> MSATSGVVNRPLVLNHGSIESTILIPTTEYHFYQTLLEGFRKSLPQVTEGFADDDEPSSKAELLMKFLGYIVQSGVSNQQEQLAAAKLVLNEFESRFLQGLNLHSYAAILLKSETFPTTLLKIKENLIKNYYLGRALVYLPGQRGLVYPPSALLNAGKSGSAQIYAIFGGQGNTDDYFEELRDIYHIYQGLVSDFVTKAQLKLQELIRTTPETDRIYTQGLDLINWLENKDKTPDQQQLLSIPMSCPLICVIQLCHYIVTCRILGITPGQLRDSLKGTTGHSQGLVTAVVVSSADSWESFEKLALQAVEFMFYIGVRGLQTYPNTSLPPSIVQDSEENAEGTPSPMLSVRDLSYDQLVKFVNETNQHLPEAKHIDISLINGPRNVVLTGPPQSLYGLNLNLRKAKAPSGLDQARIPFSERKLRFSNRFLPIMSPFHSHLLSPSTEKIVADLKKAGVEFSQSSMKLPVFDTYDGKDLRSYSGSIAARLVECITKLRVNWELSTEFNSTHVLDFGPGGASGLGVLTHRNKEGTGSRVIVAGVLDAESEDSEFGYKQEIFESNEKAIKYAPNWLKEYKPKLVKTSAGKIFVDTKFSRLLGRAPLMVPGMTPTTVSPDFVAATLNAGFHTEIAGGGYFAPSIMKAALQRVIDQVTPGTGVGINLIYVNPRMLQWGIPMIKELREQGFPIQSLSIGAGVPSLEVATEYIETLGLAHLGLKPGSIDAVNQVITIAKAHPNFPIVLQWTGGRGGGHHSFEDFHQPILQMYSKIRKCKNIILIAGSGFGSAEDTYPYLTGSWSHQFSYPSMPFDGVLFGSRVMTAKEAKTSPAAKQAIADCTGVDNSQWENTYKKPTGGIITVRSEMGEPIHKIATRGVMLWKELDDTIFTLPKNKMLEAIAKKKDYIIKKLNADYQKPWFAKNEKGTCDLEDMTYKQIAERLVELMYVRKSQRWIDVTLRNFTGKFLRRIEERFATKVGTISLIQNFSQLEEPEKAIDSVFKAYPEAASQLINEEDCDWFLLEAQSPTQKPVPFIPVLDERFEFFFKKDSLWQSE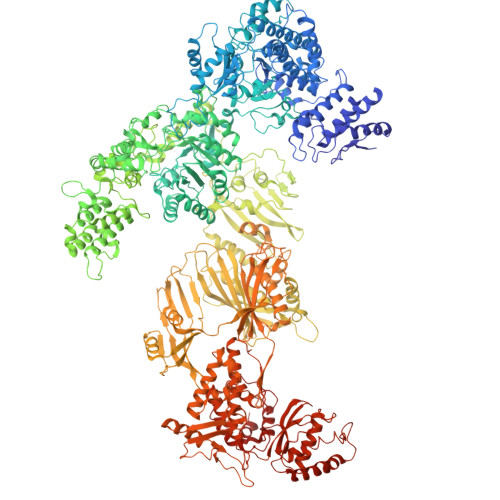DLEAVVGEDVQRTCILHGPVAAQFSNKVDEPIKDILENIHKGHIKSLVKEVYNGDESKIPVVEYFSSVDSFSDTAIEGVKIERSRNTETFTVTSGNVDNQQWFDLLAGKELSWRRAFITAARLVQGTNFVSNPAHSVLAPSKDLVVKIENGSDAKKTVLTAFQRVRGKYVPAVSLKSIGDLKIKLELIETRTADKSAVALELFYNYKPTDGFAPILEVMEGRNTSIKNFYWKLWFGSSVPVDLDFDANKPISGGEASVSSQAIAEFTHAVGNSCEDFVPRAGRPQLAPMDFAIVLGWKAIMKAIFPKTVDGDILKLVHLSNGYKMFPGADPLKKGDVVSTVAHIRSVVNGETGKTVEVVGVISRDGKPVLEVNSQFFYRGKYQDFGNSFKKTTETPVQVAFKSAKDIAVLKSKEWFHLEKDIDLLNQTLTFRCESYVKFKSSTVFASVKTTGQALLELPSKEIIQVAEINYESGSSYGNPVLDYLTRHGSTIEQPIMFENAIPLAQGTELTSKAPGTNETYAAVSGDYNPIHVNKVFASYANLPGTITHGMYSSAAVRALVEQWAAQNVATRVRAFKADFVGMVLPNDELVTHLEHVGMINGRKIIKVETKKVETEEVVLIGEAEIEQPVSTFVFTGQGSQEQGMGMDLYNSSEVAKSVWDRADVHFINNYGFSILDIVKNNPTELTVHFGGAKGRSIRNNYISMMFETVAADGQLKSEKIFKEINEDTISFTFKSPTGLLSATQFTQPALTLMEKASFEDMKSKGLVPSESMFAGHSLGEYSALTSLGDVMPIESLVDVVFYRGMTMQVAVPRDEQGRSNYGMIAVNPSRVSSTFNDSALRFVVEHIAQQTGWLLEIVNYNVENTQYVAAGDLRGLDTLSNVLNVFKIQKIDIVKLQETISLDEVKVHLSEIVDEVSKKSSSKPQPIDLERGFACIPLKGISVPFHSSYLRSGVKPFQTFLCKKIPKSAVKPANLIGKYIPNLTAKPFQLTKEYFEDVYELTKSEKIKHILDHWEEYESS>[3x]MSSKPKPIEIIGAPFSKGQPRGGVEKGPAALRKAGLVEKLKETEYNVRDHGDLAFVDVPNDSPFQIVKNPRSVGKANEQLAAVVAETQKNGTISVVLGGDHSMAIGSISGHARVHPDLCVIWVDAHTDINTPLTTSSGN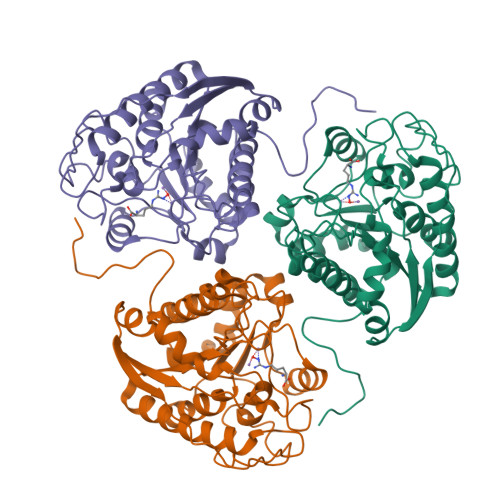LHGQPVAFLLKELKGKFPDVPGFSWVTPCISAKDIVYIGLRDVDPGEHYIIKTLGIKYFSMTEVDKLGIGKVMEETFSYLLGRKKRPIHLSFDVDGLDPVFTPATGTPVVGGLSYREGLYITEEIYKTGLLSGLDIMEVNPTLGKTPEEVTRTVNTAVALTLSCFGTKREGNHKPETDYLKPPK>MLKGKDGVVKNASTGDSIGHLQSWALDTQRDEVSGWGMGDDAERAFTTVGRASGNFEVYLDPADPSDDLEPGDLVDLELYPGGESTGSGYRSVAGALILSTAESASKDGIPMLTVNWRTSGALPQKATVS[6x];>[6x]MQFIDVEFPRDIAAGCQAVLTRRDEVVTLASGREEVNSRWADTRRSWDAGLGVRDEADLAQVVALFEEVRGRLYAFRFRDWLDWRTAATRAPITATDQPLGLGDGSRTAFQVVKVYGAVNPYTRPLSLPHPGTVRVALDGVTQPSGWTLTAPGGVITFDTPPALGVTVTAGCSFDVPVRFSDPELAVQWAYFREGQAGLAQAPSIPLIEVRLDP;>MATVLLAAAGGAIGTSLGGALFGISAAVIGQAVGGLIGQTIDARLSGGGTIKQTGPRLDSLEVMVSQEGTPLADISGRVAVAGTVIWATKLEEIARTTSTRVGSGKSSQKVKSTNFDYAASFAVSLGEGPLNGIGRIFLDGQVRDLSEMISENRVRFYPGTEDQEPDPLIEAIEGAAPAFRGTAYLVFERLFLSDFGNRVPQVRVEVFGQSGEMEKGVTGVCVIPGSTEFGYMPAPVRQQSLDGADVVWEGPENCNRYSRISDWSLSMDHLKNTLPAVQTVSLVVAWFGTDLRAGLCRFEPRIELRAKRTSIEWIAAGLNRGSATEVSRDENDRPAFGSSPADVSVVRAIMDLKARGFRVVLYPFVMMDVTADQALPSPAGTGAQGAYPWRGRIMPDVTGGRVSDQIAALMGTAQPDDFTAAVTRNKSGEISQVNLTCPGAPGDAGLRRFILHLAKLADIAGGVDAFLVGTEFRGLSQAWEPQTYADAYEFLNSSEGWFAQNAARTHEPGSLLVSATARDPRLISPPLSIDGAAARWIEIEFDRTSAPVWEGNVYYMTEDHGFAGAFRKVISDAEAPADGTRARMLLDMHDLTLGGDDWRTSTITRLRFDFSSESDAVFRIHAIRLGGGRRYPFVDALRDLAQDVDTILPTAKISYAADWSEYHSHQDAGDLTFHLDPLWADPAIDFVGIDNYLPLSDWRQGADHLDYDATSGRTTPYDLDYLKSNIEGGEYWDWFYASQEDRDTQTRTPISDGSYGEPWVFRQKAIRDWHANAHHNRTAGVRATTSTGWVPGSKPVWFTEYGCPAVDLGANRPNVFAAASSSESALPWYSSGLRDDFMQRQYLRAMAEWWTANGAPAVDLANCQAWAWDARPFPEFPLRPATWSDGPDWRLGHWLNGRAGAAPAAEAITRRAITRHGLISADIDTSRAYGQADGYAAPAPLGLGDYAQPFEVALGLQTTETGGALVIEAKPAAPLAADVIEADLVDTPAIYTLTRGALEDTPAAAIVRFRDGLSDYEITAARARIGAGKEGGSATADLALVLDGDRGNAAAEMVLRAALTSRESLSVTLPRSATTLRPGSLVEVTLGTEARRLFLVDRVVDGQAREVTLRGFDRAAYAPSGGVFKAARAGRLQGSTSSLTRFLDLPLLPGVDAPEWEGFIAAHAEPWPGAMLHSRGSTPEGSFTLAAEADARATIGRTTAALPPAPAHVWTPGPLVVTLFSGALVGRPDLDVLDGANALAIQHPDGWEVVQFREATLTADRTWRLEGLLRGQRGTDGIVGPAPLPAGAAVVAIDTALVAAGLSADDPGRALWWRSGPDAASLAAAPLRPHTFTAAGLRAFPPAHLRAVVTGGGDTSLSWVPRSRLVGTTWPDNGAPIPSGEGLERYQVTIGPTAAPVRVILADTPAATYTAAERAADGIAAPFRVAVSQISETTGPGPWIETIVTE[3x];>[3x]MTDYTDHLATGCTTLARCYILTRRDGVVMGFTDHDRDIDLDGTRCAAGAALDASTAARSLGITPDDMDAGGALSADAITEADLRAGRYDGAQVEVWEVNWTDPAVRGRLGVYTIGQVERGPLAFRAELRTRPALWNRPEGRIHTALCDVDRLGDHRCKLALGPWQSAATVIEADGADLIVSGLDETASNIFDRGVLDWTGGANAGTGSDIRVARPVAGGVRVSLWSAPPFPITAGDTANATVGCDRTADTCRNRFDNLANFRGFPLMPGESFISEYARPGDPDQSGGSRYD;>[9x]MPTPFLALPLIAEGQAGQHVTHNEALDMIDALAPRVVLSDSLATPPPAPPDRSAWIVPPGGSGFGGAGPGQIALRLGGVWHAITPAQGARWRVLDRGAAVIWSGTSWRPADVSGALGSTLGLATIEATVTATGPSVTAPALIPPRAIVLGVTSWTVQAVTGATSYRVGVPGEPDKFGASLGAAPGSSNIGVVGPFATYAPTDVVVTAEGADFTGGTIGLAASVILPGAPV

We recently characterized a novel roseophage, vB_DshS-R4C (R4C), that could infect the Dinoroseobacter shibae DFL12T, a ubiquitous group of Gram-negative α-proteobacteria of the Roseobacter clade. Here, we report the atomic capsid and in-situ structures of the tail machine of the marine siphophage, vB_DshS-R4C (R4C), which infects Roseobacter. The R4C virion, comprising 12 distinct structural protein components, has a unique five-fold vertex of the icosahedral capsid that allows genome delivery. In this study, we use cryo-electron microscopy (cryo-EM) and structure prediction to determine the atomic structure of the phage R4C capsid and the in-situ structure of the tail machinery to characterize the distinguished long rigid tail.

The distal ends of the R4C tails were re-extracted and resolved by imposing C3 symmetry, resulting in a 4.5-Å structure containing a C6 distal tail (Dit), a C3 baseplate module, and three C3 tail fibre trimers. Below the Dit is the baseplate, consisting of 3 hub proteins (vBDshSR4C_014), 3 megatron proteins (vBDshSR4C_016) and 9 fibre proteins (vBDshSR4C_017). The R4C distal tail—attaching the tail tube upward and the baseplate downward—is a C6 hexamer, as revealed by C3 reconstruction. Short loops from two adjacent monomers, and the α1 and β2-α2 loops interact with the long loop of a tail tube monomer. The Dit long loop adopts an L-shaped β-hairpin belt to create a flexible surface for optimal binding of the baseplate, mediating symmetry mismatch between the C6 Dit hexamer and the C3 megatron-hub complex. The overall R4C baseplate is homologous to that of RcGTA and both comprise hub (35.5% sequence identity), megatron (39.6% sequence identity), and fibre (30.4% sequence identity) proteins. The ion-binding domain, which comprises two discrete segments, uses four conserved Cys residues to coordinate an iron-sulfur cluster, which is essential for tail assembly and phage biological activity. The megatron protein is divided into six domains: iris/penetration (1–45), adhesion-like (46–211), peripheral, carbohydrate-binding (482–629), central (904–1130) and fibre-binding domains (1131–1447). The three α1 helices from the three megatron proteins form an iris-like gate in a closed state (inner diameter, ~10 Å) that resembles that of RcGTA36; this structure aids in preventing the eruption of genomic DNA. Each of the three tripod-like trimeric fibre complexes is formed by a combination of three tail fibre monomers, in which the head (1–35), body (36–117), and foot (118–230) regions are referred to as the rod, knob, and foot domains, respectively. Accordingly, the R4C phage equips various carbohydrate-binding accessories, including the Dit insertion domain, the megatron carbohydrate-binding and peripheral domains, the hub oligosaccharide-binding domain and the fibre foot domain to attach to the bacteria capsule.>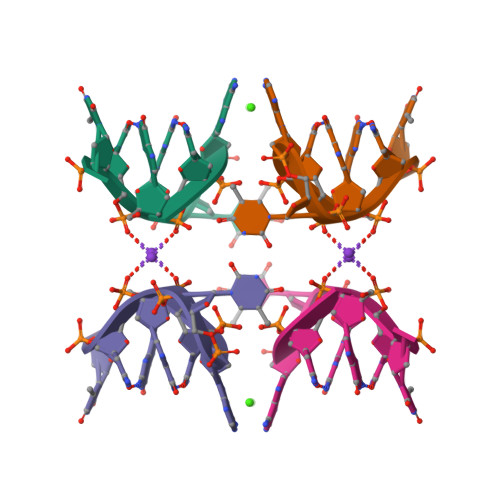 GCATGCT> MDILKLSDFIGNTLIVSLTEDRILVGSLVAVDAQM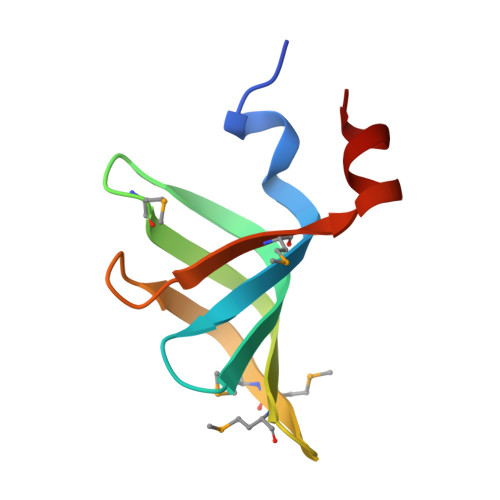NLLLDHVEERMGSSSRMMGLVSVPRRSVKTIMIDKPVLQELT Contrasting with Enterobacteria, members of the dominant genus Bacteroides often encode several BtuB vitamin B12 outer membrane transporters together with a conserved array of surface-exposed B12-binding lipoproteins. Here we show that the BtuB transporters from Bacteroides thetaiotaomicron form stable, pedal bin-like complexes with surface-exposed BtuG lipoprotein lids, which bind B12 with high affinities. Closing of the BtuG lid following B12 capture causes destabilisation of the bound B12 by a conserved BtuB extracellular loop, causing translocation of the vitamin to BtuB and subsequent transport. We propose that TonB-dependent, lipoprotein-assisted small molecule uptake is a general feature of Bacteroides spp. that is important for the success of this genus in colonising the human gut.

Here we present X-ray crystal structures of B. theta BtuG2 complexed with cyanocobalamin (the manufactured and most stable form of B12, CNCbl), adenosylcobalamin (one of the biologically active forms of vitamin B12 with the bulkiest upper ligand, AdoCbl) as well as the precursor cobinamide (Cbi), which lacks the lower ligand and the nucleotide loop. The positively charged cofactors (Co is charged +3e)20 are bound at the same site on the negatively charged face of the BtuG2 beta-propeller and make many polar and hydrophobic interactions with protein residues. To investigate whether the lack of lower ligand would affect the binding mode, we also determined the BtuG2-Cbi crystal structure, using data to 1.35 Å resolution. The orientation of the ligand is virtually the same as for the other structures, confirming BtuG2 as a versatile corrinoid binder.

> MIRVLFFIRMTMSRTIQRICLFLFCLPVFGSMGKWDYGEMEDFSVSASGLFITNEGNFQYSNATLSYYDPATCEVENEVFYRANGFKLGDVAQSMVIRDGIGWIVVNNSHVIFAIDINTFKEVGRITGFTSPRYIHFLSDEKAYVTQIWDYRIFIINPKTYEITGYIECPDMDMESGSTEQMVQYGKYVYVNCWSYQNRILKIDTETDKVVDELTIGIQPTSLVMDKYNKMWTITDGGYEGSPYGYEAPSLYRIDAETFTVEKQFKFKLGDWPSEVQLNGTRDTLYWINNDIWRMPVEADRVPVRPFLEFRDTKYYGLTVNPNNGEVYVADAIDYQQQGIVYRYSPQGKLIDEFYVGIIPGAFCWKLEHHHHHH The most abundant flagellar building block is the flagellin protein that assembles in a helical pattern of more than 20,000 copies to form the extracellular filament. Successful assembly of the flagellar filament relies on the FliS protein that prevents cytoplasmic aggregation of flagellin10 and guides flagellin to the cytoplasmic side of the fT3SS. At the fT3SS, the flagellin/FliS complex interacts with the cytoplasmic domain of the fT3SS transmembrane protein FlhA (FlhA-C). Therefore, FliS acts as targeting factor directing its flagellin client to the export gate of the fT3SS for subsequent secretion.

Multi-angle light scattering analysis indicated that the B. subtilis flagellin/FliS complex forms a heterodimer. Crystals of the flagellin/FliS complex were obtained in two spacegroups, the primitive monoclinic space group P21 at 1.5 Å resolution and the primitive orthorhombic spacegroup P22121 at 2.1 Å resolution. Notably, residues 46 to 57 are kinked by 45° in the orthorhombic structure, while the helix is straight in the crystal structure derived from monoclinic crystals. Apart from this difference, both structure superimpose well with a r.m.s.d of 1.5 over 329 Cα-atoms. The crystal structure suggests that the flagellin/FliS complex forms a rather compact particle detectable also in solution by small angle X-ray scattering (SAXS). The two proteins interact by an extensive network of hydrophobic and electrostatic interactions with an interface area of 2600 Å2 which can be divided into contact areas 1, 2 and 3. Contact area 1 involves the C-terminus of flagellin (D0-C) wrapped around the surface of FliS in an extended horseshoe like conformation with a mainly hydrophobic interaction area of 1600 Å (Contact area 1). Contact area 2 aligns FliS to the D1 core domain of flagellin, a region that was not present in previous crystal structures. Interactions within this interface are of more electrostatic nature (Contact area 2). Taken together, our crystal structure shows that the interaction between flagellin and FliS involves a complex interface at flagellin including the D1 and D0C domains.

> MRINHNIAALNTLNRLSSNNSASQKNMEKLSSGLRINRAGDDAAGLAISEKMRGQIRGLEMASKNSQDGISLIQTAEGALTETHAILQRVRELVVQAGNTGTQDKATDLQSIQDEISALTDEIDGISNRTEFNGKKLLDGTYKVDTATPANQKNLVFQIGANATQQISVNIEDMGADALGIKEADGSIAALHSVNDLDVTKFADNAADTADIGFDAQLKVVDEAINQVSSQRAKLGAVQNRLEHTINNLSASGENLTAAESRIRDVDMAKEMSEFTKNNILSQASQAMLAQANQQPQNVLQLLR;> MAIQNPYTAYQQNSVNTATPGELTLMLYNGCLKFIRLAAQAIENDDMERKNENLIKAQNIIQELNFTLNRNIELSASMGAMYDYMYRRLVQANIKNDTGMLAEVEGYVTDFRDAWKQAIQSERKDRHGSGGIA> MEKKQYLDRIKRLKERVLNTRPEMDLENAVLLTRGFKESEGQPLAIQKAYSFRKQCTEKTVKIWDDELIVGNSGSKQRGGLLNPDTCWSVLEDEIDTISERKYDPFYLTDIDRKRFNEEIKPYWKGRSTFEKWLVQIPKETKILRDCGVLYINRKAVRGWGETTAGYEMVINEGIEGIKRRIEETKNNLDITKSGHYEKLAYLKALSLVAEGIIILSKRYAKEAKRLAQLETDSKRKKELEIIAKTCDRVPEKPARTFREALQSLYFYQICIFMEQNAASYNPGRMDQYLYPYYKSDIESGRITKDEAQELLDCLWVKFSEPCLFQDEVTAQFSAGYPMFQNVCVGGIDERGMDAVNDLSFMILQATMDVQLYQPSLSVRYNMSRNSNAFLKKVAEVMKLGTGFPAFHSDEVGIQMMLNKGIPMREAYNWNPCGCVETNLAGKQRCYTSYADYNLGAIVEFVMNNGKSRKYNTQASIATGDPCTFETYNEFLGAVKNQIRYVIRAMVAGSHVNDDIGFERICPALSLSFKECISSAKDYAWGGAKYNIGNGLDAIGVADLVNSVYAVKYLVYDKKLISMEKLVKAISNDFEGYEEIQKMCLDVPKYGNDDEEVNELTADLFTFIADLIESFSGKFGHMTAGILPVSGNTPFGLEVGALPSGRNAFVPLADGVSPTAGTDIEGMGAIIKSVSHIPHIRFNQGTLLNLKLDPVFNQNANSTESLMA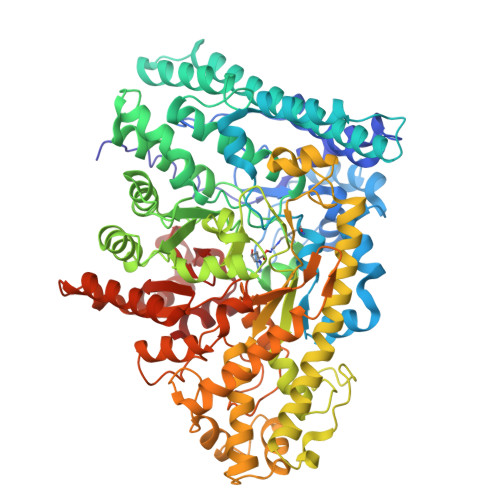FLKSMCSLGVFHVQFNVIDKEVLLDAQKHPENYKGLLIRVAGYTAYFVELGKEVQDDIIARTAHANAC> HTLVWGVWVNGVDQGDGRNIYIRSPPNNNPVKNLTSPDMTCNVDNRVVPKSVPVNAGDTLTFEWYHNTRDDDIIASSHHGPIAVYIAPAASNGQGNVWVKLFEDAYNVTNSTWAVDRLITAHGQHSVVVPHVAPGDYLFRAEIIALHEADSLYSQNPIRGAQFYISCAQITINSSDDSTPLPAGVPFPGAYTDSTP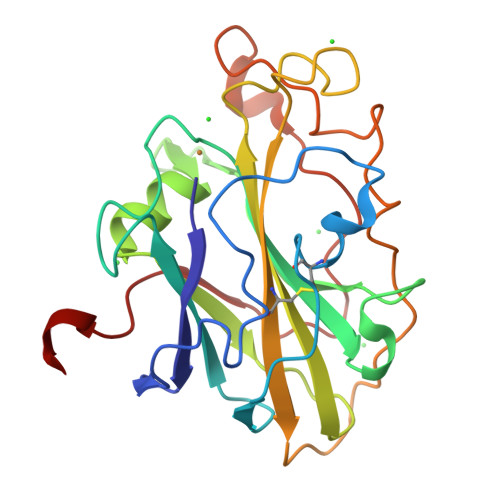GIQFNIYTTPATSYVAPPPSVWSGALGGSIAQVGDASLE>[2x]MLPHGLIVSCQALPDEP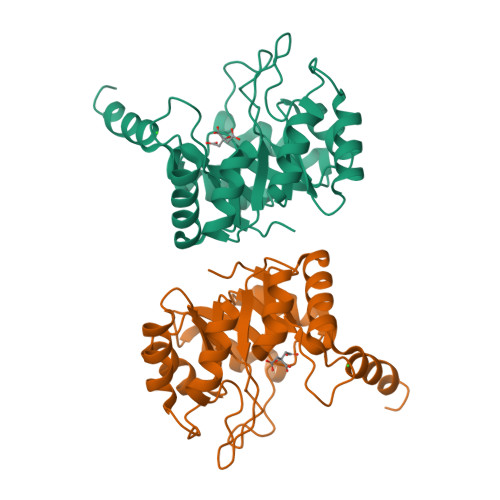LHSSFIMSKMALAAYEGGAVGIRANTKEDILAIKETVDLPVIGIVKRDYDHSDVFITATSKEVDELIESQCEVIALDATLQQRPKETLDELVSYIRTHAPNVEIMADIATVEEAKNAARLGFDYIGTTLHGYTSYTQGQLLYQNDFQFLKDVLQSVDAKVIAEGNVITPDMYKRVMDLGVHCSVVGGAITRPKEITKRFVQIMED Human NEIL1 glycosylase (hNEIL1), a bifunctional glycosylase that belongs to the Fpg/Nei family, initiates BER of a variety of DNA lesions ranging from the diastereomeric cis-5R,6S- and trans-5R,6R-dihydroxy-5,6-dihydrothymidine (thymine glycol, Tg) lesions, common oxidation damage products, to bulkier AFB1-Fapy dG lesions (22–46). Editing of pre-mRNA encoding hNEIL1 results in an amino acid change at position 242, from lysine in the unedited form of the glycosylase to arginine in the edited form. This change has been shown to modulate the rates of base excision on a range of substrates, with the unedited form being significantly more efficient in excising Tg lesions than the edited form. hNEIL1 also possesses apurinic/apyrimidinic (AP) lyase activity that catalyzes β-δ elimination, generating a single-nucleotide gap, with both 5′ and 3′ phosphates. The commonly formed diastereomeric Tg lesions may undergo hydrolytic fragmentation to form the urea lesion, N-(2-deoxy-D-erythro-pentofuranosyl)-urea.

The active site hNEIL1 mutant, CΔ100 P2G hNEIL1 (K242), was used to investigate the structural basis of urea excision. The complex that was prepared from DNA in the first eluting HPLC peak afforded a crystal that diffracted at 2.3 Å resolution. Examination of the structure revealed that the urea-modified nucleotide was extruded from the DNA and lodged in the nucleobase binding pocket employed by the glycosylase for substrate recognition and excision. When single bond distance (1.47 Å) restraints between corresponding C and N atoms were provided, the refined structure fitted better into the electron density. This indicated a covalent linkage between the Gly2 N-terminal amine and the deoxyribose C1′. The 2Fo-Fc electron density maps indicated the ring-opened deoxyribose configuration of the flipped nucleotide. Glu3 established a 2.6 Å H-bond with deoxyribose O4′, consistent with its carboxylate delivering a proton to O4′ as appeared from the merged electron density between these. The urea lesion remained covalently linked to the deoxyribose C1′ atom. The amino group of the flexible loop residue Lys242 was positioned at 3.1 and 3.6 Å from the amine and the imine of the urea moiety, respectively, suggesting the potential for H-bond formation. The void in the DNA helix created by the flipped nucleotide was stabilized by amino acids Met81, Arg118, and Phe120. We surmise that H-bonded interactions involving Glu6, Gly2 and the urea lesion may prevent subsequent proton transfer steps necessary for base excision involving Lys242, resulting in the trapping of this pre-excision complex.

> GEGPELHLASQFVNEACRALVFGGCVEKSSVSRNPEVPFESSAYRISASARGKELRLILSPLPGAQPQQEPLALVFRFGMSGSFQLVPREELPRHAHLRFYTAPPGPRLALCFVDIRRFGRWDLGGKWQPGRGPCVLQEYQQFRENVLRNLADKAFDRPICEALLDQRFFNGIGNYLRAEILYRLKIPPFEKARSVLEALQQHRPSPELTLSQKIRTKLQNPDLLELCHSVPKEVVQLGGKGYGSESGEEDFAAFRAWLRCYGMPGMSSLQDRHGRTIWFQGDPGPLAPLEHHHHHH> GSDEAAELMQQVNVLKLTVEDLEKERDFYFGKLRNIELICQENEGENDPVLQRIVDIL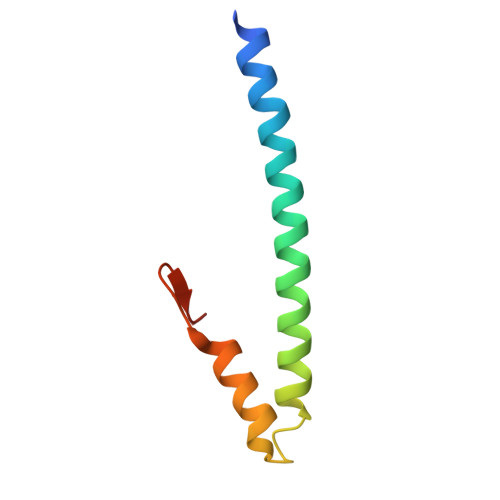YATDEGFVIPDEGG> SLLTCGGCQQNIGDRYFLKAIDQYWHEDCLSCDLCGCRLGEV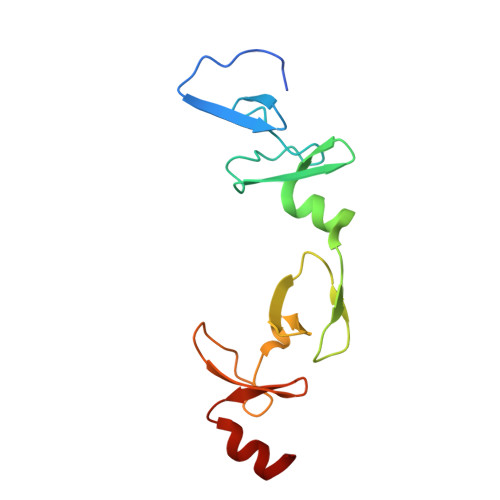GRRLYYKLGRKLCRRDYLRLFGQDGLCASCDKRIRAYEMTMRVKDKVYHLECFKCAACQKHFCVGDRYLLINSDIVCEQDIYEWTKING> MVSLPRMVYPQPK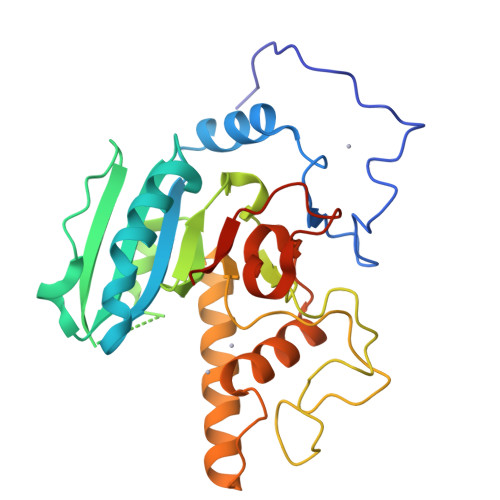VLTPCRKDVLVVTPWLAPIVWEGTFNIDILNEQFRLQNTTIGLTVFAIKKYVAFLKLFLETAEKHFMVGHRVHYYVFTDQPAAVPRVTLGTGRQLSVLEVGAYKRWQDVSMRRMEMISDFCERRFLSEVDYLVCVDVDMEFRDHVGVEILTPLFGTLHPSFYGSSREAFTYERRPQSQAYIPKDEGDFYYMGTFFGGSVQEVQRLTRACHQAMMVDQANGIEAVWHDESHLNKYLLRHKPTKVLSPEYLWDQQLLGWPAVLRKLRFTAVPKNHQAVRNP2-[5-(6-METHYLPYRIDIN-2-YL)-2,3-DIHYDRO-1H-PYRAZOL-4-YL]-1,5-NAPHTHYRIDINE | C17 H15 N5 | 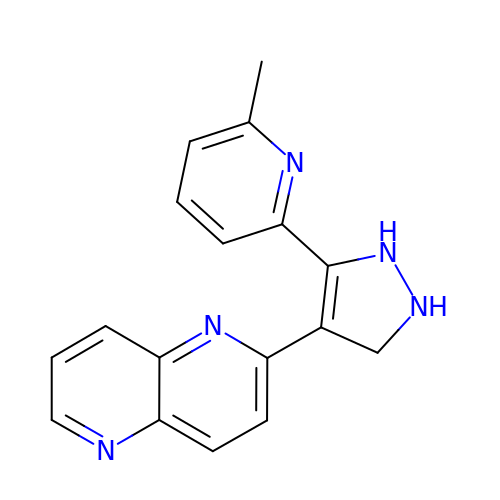YRBHUKMLAGQYHS-UHFFFAOYSA-N> TVAYIAIGSNLASPLEQVNAALKALGDIPESHILTVSSFYRTPPLGPQDQPDYLNAAVALETSLAPEELLNHTQRIELQQGRVRKAERWGPRTLALDIMLFGNEVINTERLTVPHYDM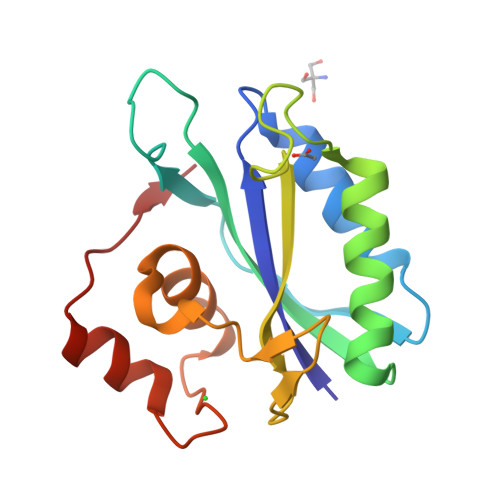KNRGFMLWPLFEIAPELVFPDGEMLRQILHTRAFDKLNKW>[4x]MIRYLRGLVLKKEAGGFVLLAGGVGFFLQAPTPFLQALEEGKEVGVHTHLLLKEEGLSLYGFPDEENLALFELLLSVSGVGPKVALALLSALPPRLLARALLEGDARLLTSASGVGRRLAERIALELKGKVPPHLLAGEK

In bacteria, RuvA, RuvB, and RuvC are involved in processing the HJ. RuvA was shown to assemble into a tetramer for recognizing the HJ core and recruits RuvB. As a motor protein, RuvB can bind the dsDNA part of the HJ and promote the movement of HJ, known as branch migration. RuvB belongs to the AAA+ (ATPase associated with various cellular activities) family, which includes many members involved in numerous physiological processes.

To understand the mechanisms of RuvB recruitment to the HJ DNA by RuvA, we reconstituted the complex of RuvA-RuvB-HJ DNA for structural analysis. To our surprise, we only obtained a structure of RuvA-HJ DNA. Perhaps, the entire complex readily dissociated during grid preparation. Cryo-EM structure of the RuvA-HJ DNA complex revealed that RuvA assembles as a tetramer to recognize the crossover of HJ DNA through charge-charge interactions, which is consistent with previous biochemical and structural analysis. A crystal structure of RuvA in complex with HJ has revealed that RuvA forms a unique tetrameric architecture, in which domains I and II are responsible for Holliday junction binding. Lastly, RuvB is loaded onto HJ DNA by interacting with RuvA, which assembles as a tetramer to bind to the HJ core.(E)-3-((5,6-dihydro-2H,4H-thiazolo[5,4,3-ij]quinolin-2-ylidene)amino)-2-hydroxy-1-(4-(isoquinolin-5-yl)piperazin-1-yl)-2-methylpropan-1-one | C27 H29 N5 O2 S | 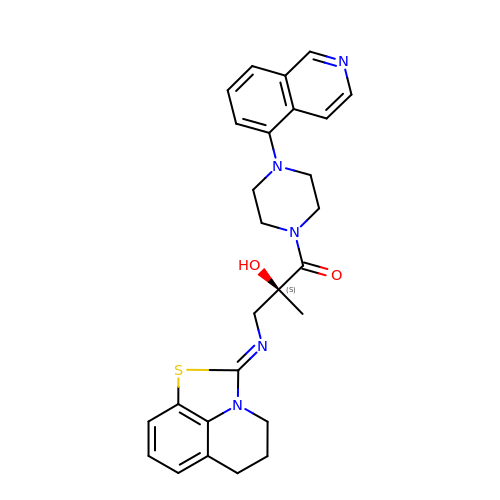QZFUDKGJJOEDLX-PTRKPBRWSA-N4-[2,4-bis(oxidanylidene)-6-(trifluoromethyl)-1H-pyrimidin-3-yl]-5-methoxy-2-(2-methylphenoxy)benzenecarbonitrile | C20 H14 F3 N3 O4 | 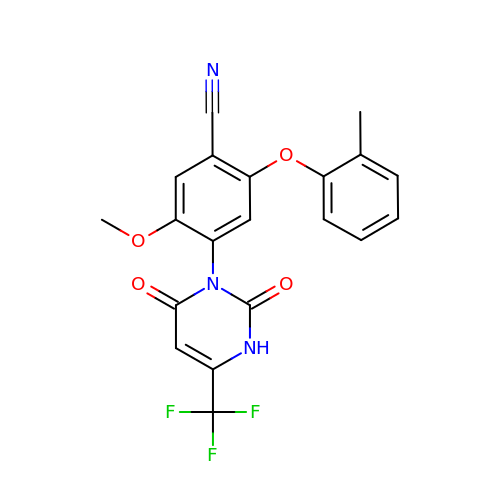GSEHYSQYWAECFH-UHFFFAOYSA-N>LPTSNPAQELEARQLGRTTRDDLINGNSASCADVIFIYARGSTETGNLGTLGPSIASNLESAFGKDGVWIQGVGGAYRATLADNFLPRGTSSAAIREMLGLFQQANTKCPDATLIAGGYSQGAALAAASIEDLDSAIRDKIAGTVLFGYTKNLQNRGRIP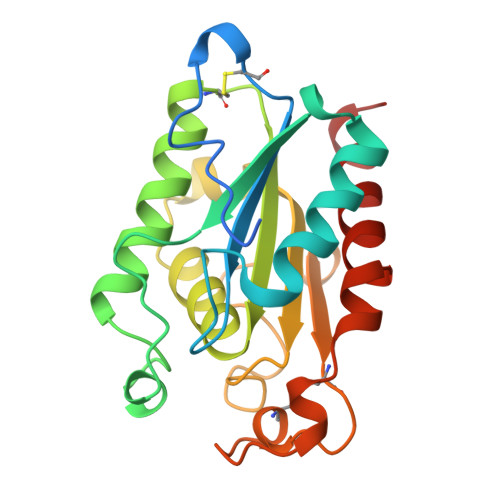NYPADRTKVFCNTGDLVCTGSLIILAPHFAYGPDARGPAPEFLIEKVRAVRGSA[2x]2C-methyl-D-erythritol-2,4-cyclodiphosphate synthase (IspF) catalyzes the conversion of 4-diphosphocytidyl-2C-methyl-D-erythritol-2-phosphate to 2C-methyl-D-erythritol-2,4-cyclodiphosphate and cytidine monophosphate in production of isoprenoid-precursors via the methylerythritol phosphate biosynthetic pathway. IspF represents a potential target for development of broad-spectrum antimicrobial drugs since it is proven or inferred as essential in these pathogens and absent from mammals. In all IspF crystal structures three subunits form a compact bell-shaped assembly approximately 45 Å by 60 Å in the axial and equatorial dimensions respectively. The enzyme active site is located in a cleft at the interface of two subunits and here Zn2+ is coordinated by the side chains of two histidines and an aspartate.

Surprisingly, a second molecule of CMP was observed in the active site when BcIspF was co-crystallized in the presence of 10 mM ligand. This second CMP is likely due to the high concentration used and represents an artifact of crystallization, unlikely to have physiological significance. The binding of CMP 2 within the three active sites of the asymmetric unit is very similar, for example the main chain conformation of the α2-α3 loop and the positions of Leu78 and His36 interacting with van der Waals forces on either side of the pyrimidine and helping to position it is essentially the same. In addition the position of Phe63 that helps to position Leu78 is also conserved. However, there are differences in the orientation of two side chains that change the detail of the hydrogen bonding interactions with CMP 2. In active site A two solvent mediated links are noted involving the carbonyl groups of Ser64, Phe70 and Ala73 and cytosine O2 and N3. Overlay with the EcIspF-product complex shows that CMP 2 binds in the same location as MEcPP and indeed exploits interactions with the same residues, the majority of which are conserved. The binding pose of CMP 2 offers clues about molecular features that might be considered for ligand design targeting this area of the active site. The unexpected observations that a second molecule of CMP can occupy the active site as well as the presence of citrate interacting with Zn2+ in BcIspF are noteworthy.

>[3x]MGSSHHHHHHSSGENLYFQGHMDVRIGQGYDVHQLVEGRPLIIGGVTIPYERGLLGHSDADVLLHAITDALFGAAALGDIGRHFSDTDAAFKGADSRVLLRACAERVKAAGFTIQNVDSTVIAQAPKLAPHIDGMRANIAADLGLPLERVNVKAKTNEKLGYLGRGEGIEAQAAALLVKQGG> MNGSADAGPRPRKYVFITGGVVSSLGKGILTSSLGALLRARGYRVTAIKIDPYVNVDAGTMRPYEHGEVFVTADGAETDLDIGHYERFLDMDLSRGNNLTTGQVYLSVIQKERRGEYLSQTVQVIPHITDEIKERIRKVAEEQKAEIVVVEVGGTVGDIESLPFLEAIRQFRFDEGEGNTLYLHLTLVPYLETSEEFKTKPTQHSVATLRGVGIQPDILVLRSARPVPEEVRRKVALFTNVRPGHVFSSPTVEHLYEVPLLLEEQGLGRAVERALGLEA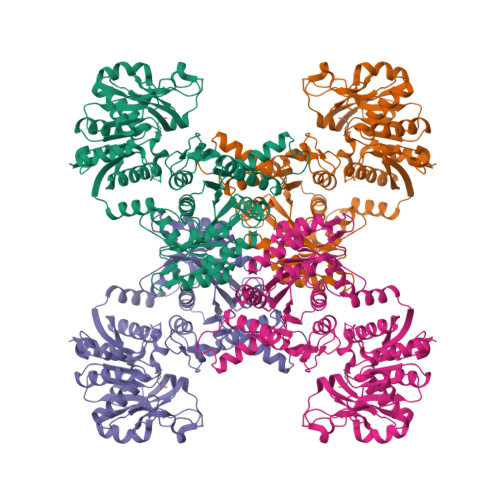VIPNLSFWQEAVRVLKHPERTVKIAIAGKYVKMPDAYLSLLEALRHAGIKNRARVEVKWVDAESLEAADLEEAFRDVSGILVPGGFGVRGIEGKVRAAQYARERKIPYLGICLGLQIAVIEFARNVAGLKGANSTEFDPHTPHPVIDLMPEQLEVEGLGGTMRLGDWPMRIKPGTLLHRLYGKEEVLERHRHRYEVNPLYVDGLERAGLVVSATTPGMRGRGAGLVEAIELKDHPFFLGLQSHPEFKSRPMRPSPPFVGFVEAALAYQERA>[2x]MTLLGTALRPAATRVMLLGSGELGKEVAIECQRLGVEVIAVDRYADAPAMHVAHRSH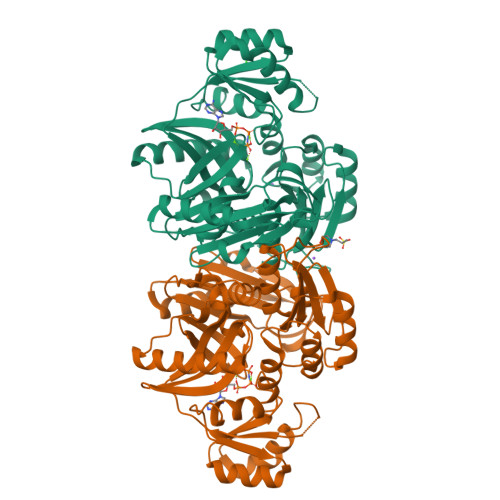VINMLDGDALRRVVELEKPHYIVPEIEAIATDMLIQLEEEGLNVVPCARATKLTMNREGIRRLAAEELQLPTSTYRFADSESLFREAVADIGYPCIVKPVMSSSGKGQTFIRSAEQLAQAWKYAQQGGRAGAGRVIVEGVVKFDFEITLLTVSAVDGVHFCAPVGHRQEDGDYRESWQPQQMSPLALERAQEIARKVVLALGGYGLFGVELFVCGDEVIFSEVSPRPHDTGMVTLISQDLSEFALHVRAFLGLPVGGIRQYGPAASAVILPQLTSQNVTFDNVQNAVGADLQIRLFGKPEIDGSRRLGVALATAESVVDAIERAKHAAGQVKVQG4-({6-AMINO-5-BROMO-2-[(4-CYANOPHENYL)AMINO]PYRIMIDIN-4-YL}OXY)-3,5-DIMETHYLBENZONITRILE | 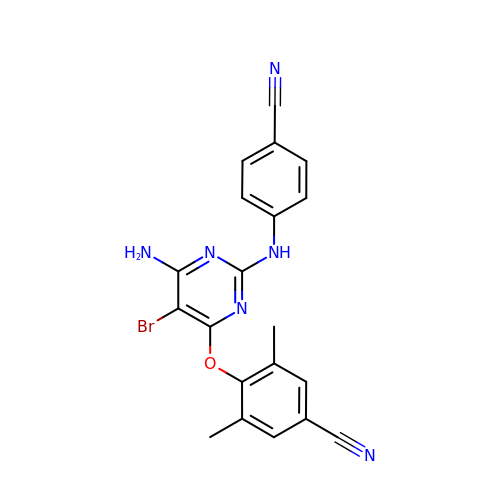C20 H15 Br N6 O | PYGWGZALEOIKDF-UHFFFAOYSA-N>ARTVVLITGCSSGIGLHLAVRLASDPSQSFKVYATLRDLKTQGRLWEAARALACPPGSLETLQLDVRDSKSVAAARERVTEGRVDVLVCNAGLGLLGPLEALGEDAVASVLDVNVVGTVRMLQAFLPDMKRRGSGRVLVTGSVGGLMGLPFNDVYCASKFALEGLCESLAVLLLPFGVHLSLIECGPVHTAFMEKVLGSPEEVLDRTDIHTFHRFYQYLALSKQVFREAAQNPEEVAEVFLTALRAPKPTLRYFTTERFLPLLRMRLDDPSGSNYVTAMHREVFGDVPAKAEAGAEAGGGR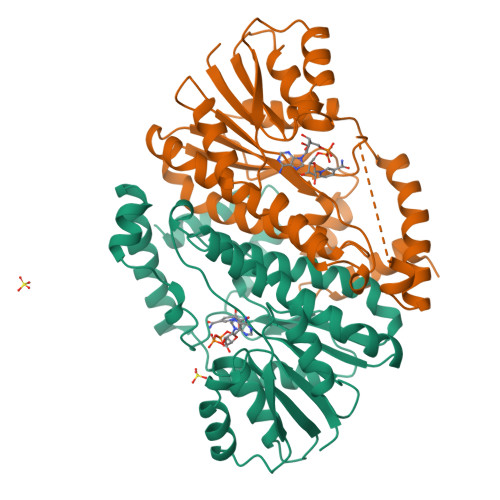GPGAEDEAGRSAVGDPELGDPPAAPQ[4x]> MGSSHHHHHHSSGENLYFQGGTMYDFEYLNGLSYTELTNLIKNIKWNQINGLFNYSTGSQKFFGDKNRVQAIINALQESGRTYTANDMKGIETFTEVLRAGFYLGYYNDGLSYLNDRNFQDKCIPAMIAIQKNPNFKLGTAVQDEVITSLGKLIGNASANAEVVNNCVPVLKQFRENLNQYAPDYVKGTAVNELIKGIEFDFSGAAYEKDVKTMPWYGKIDPFINELKALGLYGNITSATEWASDVGIYYLSKFGLYSTNRNDIVQSLEKAVDMYKYGKIAFVAMERITWDYDGIGSNGKKVDHDKFLDDAEKHYLPKTYTFDNGTFIIRAGDKVSEEKIKRLYWASREVKSQFHRVVGNDKALEVGNADDVLTMKIFNSPEEYKFNTNINGVSTDNGGLYIEPRGTFYTYERTPQQSIFSLEELFRHEYTHYLQARYLVDGLWGQGPFYEKNRLTWFDEGTAEFFAGSTRTSGVLPRKLILGYLAKDKVDHRYSLKKTLNSGYDDSDWMFYNYGFAVAHYLYEKDMPTFIKMNKAILNTDVKSYDEIIKKLSDDANKNTEYQNHIQELVDKYQGAGIPLVSDDYLKDHGYKKASEVYSEISKAASLTNTSVTAEKSQYFNTFTLRGTYTGETSKGEFKDWDEMSKKLDGTLESLAKNSWSGYKTLTAYFTNYRVTSDNKVQYDVVFHGVLTDNG

Clostridial collagenases are among the most efficient enzymes to degrade by far the most predominant protein in the biosphere. Clostridia employ collagenases for nutrition (e.g. saprophytic strains) and host colonization (1–3). They are large multidomain proteins of ∼115 kDa belonging to the gluzincin superfamily of metalloproteases. Here we present the crystal structures of the peptidase domains of ColH and ColT and the collagenase unit of ColG in the presence and absence of the peptidic inhibitor isoamylphosphonyl-Gly-Pro-Ala bound to the active site.

The recently determined crystal structure of ColG revealed a saddle-shaped architecture with a distinct segmentation of the N-terminal collagenase unit. The collagenase unit is capable of degrading native collagen in the absence of the accessory domains within the C-terminally located collagen recruitment unit in vitro. The comparison of the isolated peptidase domains of ColH and ColT with the crystal structure of ColG containing the full collagenase unit plus the PKD-like domain reveals that the peptidase structure is unaffected by the contiguous domains. Although all peptidases adopted an open conformation in the unliganded apo-form and a more compact conformation in the complexed state, this breathing movement was most pronounced in ColG and least pronounced in ColH. Near the S5 site defined by the edge strand (Pro499) and ∼15 Å apart from the catalytic zinc, we could identify a structurally conserved calcium binding site. In the ColG crystal structures, this site remained unloaded because of the presence of at least 125 mm citrate in the crystallization buffer. As evidenced by the comparison of Ca2+-unloaded (ColG) and -loaded (ColH/T) crystal structures, the liganding glutamate side chain undergoes a marked rearrangement upon Ca2+ binding that allows Ca2+ coordination. The crystal structure analysis of ColG suggested that N-terminally extended substrates assist in their hydrolysis by employing additional interactions with the edge strand in ColG. The interaction areas between the inhibitor isoamylphosphonyl-GPA with the individual enzymes is largest in ColH (256 Å2) > ColT (248 Å2) > ColG (220 Å2), as calculated using the PISA server. This relation explains the need of ColG for N-terminally extended peptides to obtain full peptidolytic activity.>MGSSHHHHHHSSGLVPRGSMAAPFDKSKNVAQSIDQLIGQTPALYLNKLNNTKAKVVLKMECENPMASVKDRLGFAIYDKAEKEGKLIPGKSIVVESSSGNTGVSLAHLGAIRGYKVIITMPESMSLERRCLLRIFGAEVILTPAALGMKGAVAMAKKIVAANPNAVLADQFATKYNALIHEETTGPEIWEQTNHNVDCFIAGVGTGGTLTGVARALKKMGSHARIVAVEPTESPVLSGGKPGPHKIQGIGPGFVPDVLDRSLIDEVLCVAGDDAIETALKLTRSDGVFCGFSGGANVYAALKIAERPEMEGKTIVTVIPSFGERYLSTTLYRSVRDEVSSLPVVDASELQD[2x]

The de novo pathway of cysteine biosynthesis requires the conversion of O-acetyl-l-serine into l-cysteine, which is catalysed by cysteine synthase (CS). As CS is not found in humans, it constitutes a potential drug target. Crystal structures of the three enzymes were determined at resolutions of 1.80 Å for TcCS, 1.75 Å for LiCS and 2.75 Å for TthCS. These three homodimeric structures show the same overall fold and demonstrate that the active-site geometry is conserved, supporting a common reaction mechanism.

Each LiCS monomer adopts a compact structure composed of nine α-helices and 12 β-sheets with an extended C-terminal tail. The C-terminal tail of each chain is formed by a flexible region that stretches across to the partner subunit of each dimer, forming an extensive interface. Further analysis of the homodimer with PISA shows that LiCS has a large dimer interface involving 27.0% of chain A residues and 26.6% of chain B residues. The active site of LiCS is found at the centre of each subunit between α1 and α5. Although the purified protein was yellow in colour, suggesting the presence of the cofactor PLP, no electron density for the cofactor was observed. It is likely that the PLP was lost during crystallization. As no PLP was identified at the active-site lysine of LiCS, this conformation corresponds to the apo form of the enzyme. The structure of LiCS was resolved in the open apo form, showing key changes when PLP is not bound to the active site, specifically the absence of a loop covering the active site. In comparison, under the conditions of the assay LiCS produces significantly higher concentrations of cysteine than TcCS and TthCS, reaching 2 mM cysteine before plateauing at 5 mM OAS.> VLGGGAIYGGGSRCSAAFNVTK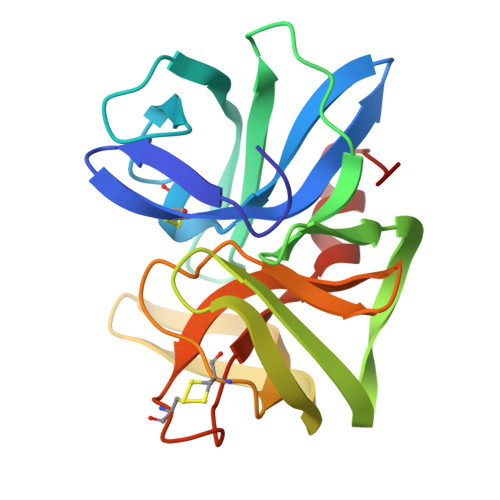GGARYFVTAGHCTNISANWSASSGGSVVGVREGTSFPTNDYGIVRYTDGSSPAGTVDLYNGSTQDISSAANAVVGQAIKKSGSTTKVTSGTVTAVNVTVNYGDGPVYNMVRTTACSAGGDSGGAHFAGSVALGIHSGSSGCSGTAGSAIHQPVTEALSAYGVTVY> MSSRLLPPNRSSLERSLGDVLPAELPVPLRELHDPARCEAALLPYLAWTRSVDR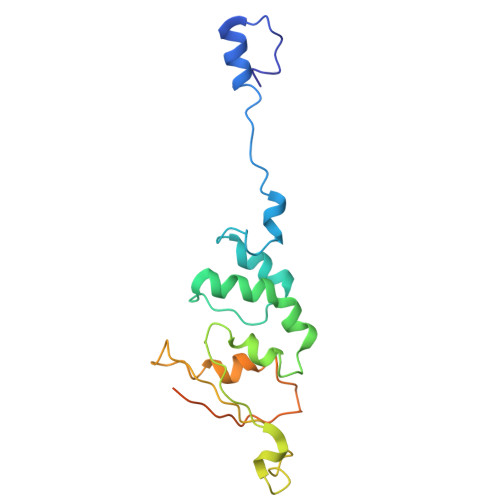WDPDWSDEAKRNAVATSFVLHQRKGTLTALRQVVEPIGALSEVTEWWQRSPTGVPGTFEITVDVSDRGIDEGTVLELERLLDDVRPVSRHLTRLDLRITPVIRSRHGLAVTDGDTLEIFPWKQ> ALWQFNGMIKCKIPSSEPLLDFNNYGCYCGLGGSGTPVDDLDR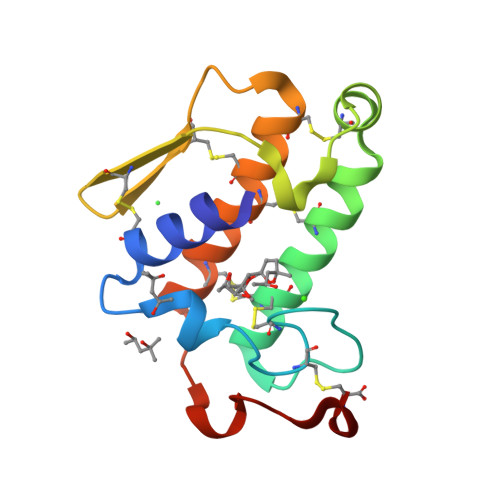CCQTHDNCYKQAKKLDSCKVLVDNPYTNNYSYSCSNNEITCSSENNACEAFICNCDRNAAICFSKVPYNKEHKNLDKKNC>[12x]SNADASTDLQNRLSKVNSFHASFSQAVTSSDGAVVQEGEGELW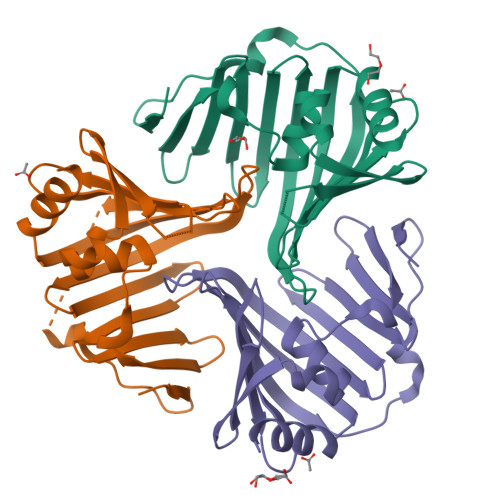VKRPNLFNWHMTSPDESVLISDGETLWFYNPFVEQATATWLKNATGNTPFMLITRNNPDDWKQYNVKQKGDDFELTPKSASGNLKQFAISVTPSGTIKSFTAVEQDGQRSAYTLKSQQSSVVDASKFTFTPPKGVTLDDQR>[2x]GS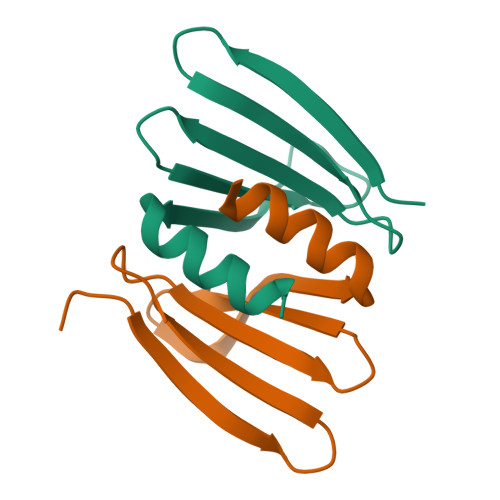GLNIKENDLPGIGKKFEIETRSHEKMTIIIHDDGRREIYRFNDRDPDELLSNISLDDSEARQIAAILGG> MVPISPIETVPVKLKPGMDGPKVKQWPLTEEKIKALVEICTEMEKEGKISKIGPENPYNTPVFAIKKKDSTKWRKLVDFRELNKRTQDFWEVQLGIPHPAGIKKNKSVTVLDVGDAYFSVPLDEDFRKYTAFTIPSINNETPGIRYQYNVLPQGWKGSPAIFQSSMTKILEPFAAQNPDIVIYQYMDDLYVGSDLEIGQHRTKIEELRQHLLRWGLTTPDKKHQKEPPFLWMGYELHPDKWTVQPIVLPEKDSWTVNDIQKLVGKLNWASQIYPGIKVRQLSKLLRGTKALTEVIPLTEEAELELAENREILKEPVHGVYYDPSKDLIAEIQKQGQGQWTYQIYQEPFKNLKTGKYARMRGAHTN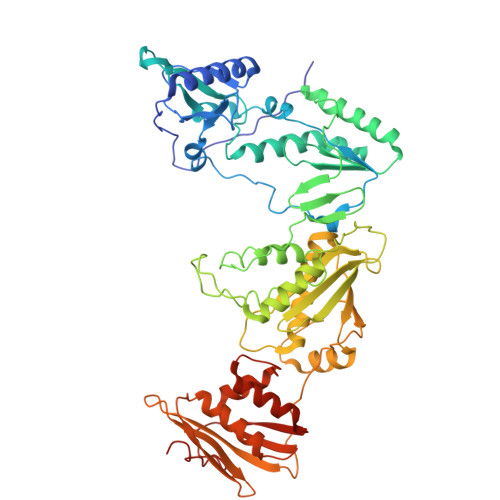DVKQLTEAVQKITTESIVIWGKTPKFKLPIQKETWETWWTEYWQATWIPEWEFVNTPPLVKLWYQLEKEPIVGAETFYVDGAANRETKLGKAGYVTNKGRQKVVPLTNTTNQKTELQAIYLALQDSGLEVNIVTDSQYALGIIQAQPDKSESELVNQIIEQLIKKEKVYLAWVPAHKGIGGNEQVDKLVSAG HUH endonucleases are diverse enzymes that contain an eponymous motif consisting of a pair of conserved metal-coordinating histidine (H) separated by a bulky hydrophobic residue (U). Replication-initiating HUH endonucleases (Reps) are sequence-specific nucleases that cleave and rejoin single-stranded DNA (ssDNA) during rolling-circle replication. Replication initiator proteins (Reps) from this HUH endonuclease superfamily are found in a variety of bacterial plasmids and viral genomes, including circular Rep-encoding single-stranded DNA (CRESS-DNA) viruses that are known to infect organisms across all three domains of life (1–5). These enzymes initiate rolling-circle replication through sequence-specific processing of the viral single-stranded DNA (ssDNA) genome via cleavage and subsequent phosphotyrosine covalent linkage to the ssDNA’s newly exposed 5′ end. Following linkage, the genome’s freed 3′-OH can be used as a primer for DNA replication before its ultimate return to the active site, where it attacks the phosphotyrosine intermediate to rejoin and release the circular ssDNA genome.

To better understand the roles that coordinated divalent ions play in Rep function, we resolved two cocrystal structures of the endonuclease domain of DCV Rep in complex with a cognate ssDNA 10-mer (5′-TATTATTACC-3′) derived from the DCV Ori, with and without manganese coordinated in the active site. Precleavage complexes were obtained using the dDCV mutant. The substrate in both structures conforms to the characteristic “U”-shaped architecture, indicating that the ssDNA conformation is largely facilitated by the DNA binding interface and intramolecular base pairing and base stacking, with little support from the coordinated cation. In the DCV plus Mn2+ structure, the Mn2+ is coordinated by His52 and Gln54 within the HUQ motif along with the third residue of the coordinating triad Glu44, and a water, which, in turn, is positioned by Glu95. Two hydrogen bonds from the scissile phosphate complete the octahedral coordination of Mn2+. A conserved Lys94 is oriented toward the catalytic residue and facilities a hydrogen bond with the scissile phosphate, adding evidence that this lysine may not only be a general base but that it might also play a cooperative structural role with the ion in stabilizing the ssDNA backbone in the active site. In further comparisons of these two structures, we noticed the ssDNA substrate seemed to be positioned much farther into the active site in the presence of Mn2+. In the absence of Mn2+, the measured distance is 3.0 Å, whereas when Mn2+ is coordinated in the active site, and the scissile phosphate is pulled 0.7 Å closer to the oxygen, with a measured distance of 2.3 Å. Considering that Mn2+ coordination includes two ion-dipole bonds with the scissile phosphate, it is likely this is the driving force behind bringing the tyrosine in close proximity to the phosphate.

> MAKSGNYSYKRWVFTINNPTFEDYVHVLEFCTLDNCKFAIVGEEKGANGTPHLQGFLNLRSNARAAALEESLGGRAWLSRARGSDEDNEEFCAKESTYLRVGEPVSKGRSS>AMAQIDLNITCRFAGVFHVEKNGRYSISRTEAADLCKAFNSTLPTMAQMEKALSIGFETCRYGFIEGHVVIPRIHPNSICAANN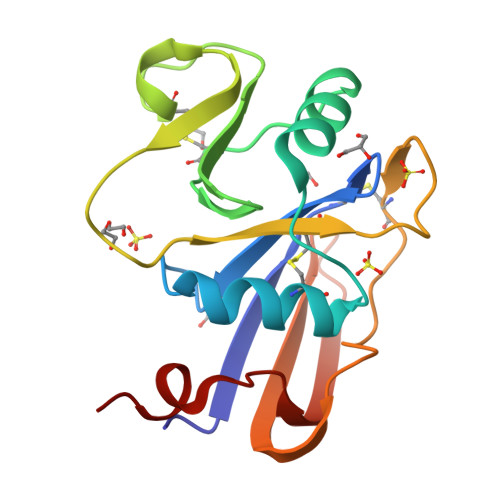TGVYILTSNTSQYDTYCFNASAPPEEDCTSVTDLPNAFDGPITITIVNRDGTRYVQKGEYRTNPEDIYPS[2x]> RNFNNLTKGLCTINSWHIYGKDNAVRIGESSDVLVTREPYVSCDPDECRFYALSQGTTIRGKHSNGTIHDRSQYRALISWPLSSPPTVYNSRVECIGWSSTSCHDGKSRMSICISGPNNNASAVVWYNRRPVAEINTWARNILRTQESECVCHNGVCPVVFTDGSATGPADTRIYYFKEGKILKWESLTGTAKHIEECSCYGERTGITCTCKDNWQGSNRPVIQIDPVAMTHTSQYICSPVLTDNPRPNDPNIGKCNDPYPGNNNNGVKGFSYLDGANTWLGRTISTASRSGYEMLKVPNALTDDRSKPIQGQTIVLNADWSGYSGSFMDYWAEGD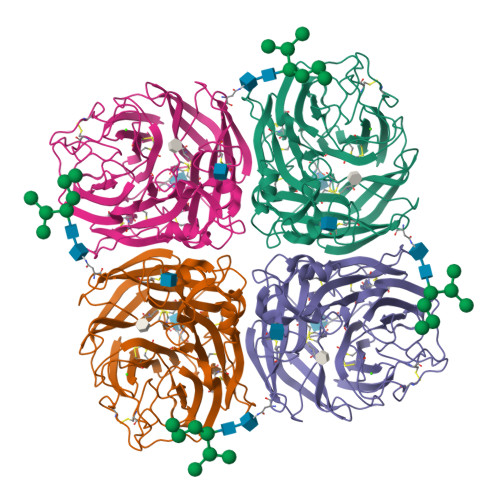CYRACFYVELIRGRPKEDKVWWTSNSIVSMCSSTEFLGQWNWPDGAKIEYFL> GSHMASMKPIFDINETFEKQLKDLTSNVKSIQDNLLEEIITPNTKTEYLQRFLIDRFDKELFKKNVPIVSYEDIKPYLDRVVNGESSDVISARTITGFLLSSGTSGGAQKMMPWNNKYLDNLTFIYDLRMQVITKHVKGVEEGKGMMFLFTKQESMTPSGLPARVATSSYFKSDYFKNRPSNWYYSYTSPDEVILCPNNTESLYCHLLCGLVQRDEVVRTGSIFASVMVRAIEVLKNSWEELCSNIRSGHLSNWVTDLGCQNSVSLVLGGPRPELADTIEEICNQNS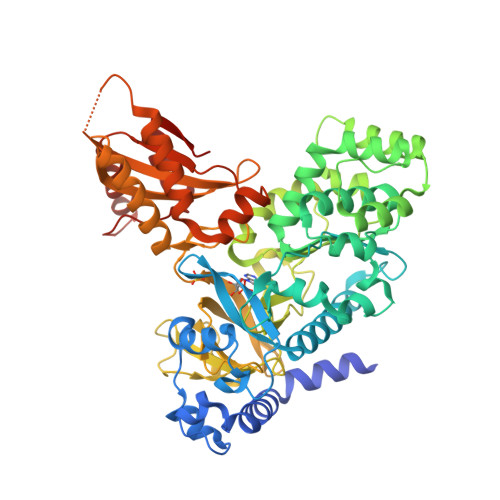WKGIVKRLWPNTKYIETVVTGSMGQYVPMLNYYCNDLPLVSTTYGSSETTFGINLDPLCKPEDVSYTFMPNMSYFEFIPMDGGDKNDVVDLEDVKLGCTYEPVVTNFAGLYRMRVGDIVLVTGFYNNAPQFKFVRRENVVLSIDSDKTNEEDLFKAVSQAKLVLESSGLDLKDFTSYADTSTFPGHYVVYLEVDTKEGEEKETAQFELDEEALSTCCLVMEESLDNVYKRCRFKDGSIGPLEIRVVRQGTFDSLMDFFISQGASTGQYKTPRCIKSGKALQVLETCVVAKFFSI> MGKEKTHINIVVIGHVDSGKSTTTGHLIYKCGGIDKRTIEKFEKEAAEMGKGSFKYAWVLDKLKAERERGITIDISLWKFETTKYYITIIDAPGHRDFIKNMITGTSQADCAVLIVAAGVGEFEAGISKNGQTREHALLAYTLGVKQLIVGVNKMDSTEPAYSEKRYDEIVKEVSAYIKKIGYNPATVPFVPISGWHGDNMLEPSPNMPWFKGWKVERKEGNASGVSLLEALDTILPPTRPTDKPLRLPLQDVYKIGGIGTVPVGRVETGILRPGMVVTFAPVNITTEVKSVEMHHEAL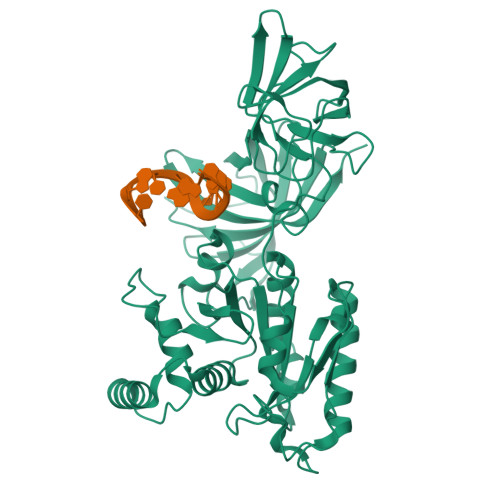SEALPGDNVGFNVKNVSVKDIRRGNVCGDSKSDPPQEAAQFTSQVIILNHPGQISAGYSPVIDCHTAHIACKFAELKEKIDRRSGKKLEDNPKSLKSGDAAIVEMVPGKPMCVESFSQYPPLGRFAVRDMRQTVAVGVIKNVEKKSGGAGKVTKSAQKAQKAGK To provide easy-to-use automated NCS restraints, it was decided to adopt a different approach that uses interatomic distances rather than structural superposition, extending the ideas used in the SHELX program. The restraints encourage NCS-related chains to have similar local structure, but differences are allowed to occur at a fixed cost. The restraints can also be used for another commonly encountered case of molecular similarity, namely that to a separate already determined structure that remains fixed during the refinement of the structure being refined.

In using LSSR target restraints it is sensible to ensure that the high-resolution target structure has as good a structure as possible.

> ACDYTCGSNCYSSSDVSTAQAAGYQLHEDGETVGSNSYPHKYNNYEGFDFSVSSPYYEWPILSSGDVYSGGSPGADRVVFNENNQLAGVITHTGASGNNFVECT Here, we report the biochemical and structural characterisation of a third esterase from the A. fulgidus genome, named AF-Est2 (locus tag: AF1537). This belongs to the α/β hydrolase 6 family and the X group of the ESTHER classification. AF-Est2 was tested against a range of p-nitrophenyl (pNP) esters and was shown to be active against small to medium acyl chain length esters (C2 to C8), which is consistent with its classification as an esterase rather than a lipase.

The structure has been isotropically refined to a resolution of 1.4 Å with a final Rfree of 17.5. The structure reveals, as expected, a canonical α/β hydrolase fold core domain (Asp1-Arg117 and Asp176-His254), and a cap domain (Leu118-Phe175) formed by helices α5-α8. The active site is located at the interface of the core and the cap domains with the conserved catalytic triad composed of Ser89, His228 and Asp200. The structure also contains two CoA molecules at full occupancy, several ordered PEG molecules and a single citrate molecule bound at a crystal contact. The AF-Est2 esterase structure has shown a novel binding mode for a CoA molecule which is located in a groove overlapping the active site of the enzyme where the pantetheine moiety is partially obstructing the alcohol binding pocket. There is an ion pair formed by the diphosphate moiety of the CoA and the guanidinium group of Arg117. The adenine ring of CoA is stacked in a pocket between the side chains of Tyr207 and Leu178 and its N6A atom makes a H-bond to the main chain oxygen of Arg117. However high activity of AF-Est2 towards the pNP esters suggests that the flexible CoA pantetheine group is displaced from the alcohol pocket upon substrate binding. The necessity of the CoA pantetheine group displacement for pNP ester hydrolysis was confirmed by incubation of the AF-Est2 with the disulfide inducing agent diamide which enforces the formation of a covalent bond between the thiol groups of CoA and Cys172. This oxidised enzyme shows no activity towards pNP-valerate demonstrating that this enzyme is inhibited by the formation of the disulfide.

>MLERVFIDVDGVKVSLLKGRERKVFYIHSSGSDATQWVNQLTAIGGYAIDLPNHGQSDTVEVNSVDEYAYYASESLKKTVGKAVVVGHSLGGAVAQKLYLRNPEICLALVLVGTGARLRVLPEILEGLKKEPEKAVDLMLSMAFASKGEEYEKKRREFLDRVDVLHLDLSLCDRFDLLEDYRNGKLKIGVPTLVIVGEEDKLTPLKYHEFFHKHIPNSELVVIPGASHMVMLEKHVEFNEALEKFLKKVGVAEVHHHHHH[2x]(4S)-3-methyl-5,6,7,8-tetrahydro[1,2,4]triazolo[4,3-a]pyrazine | C6 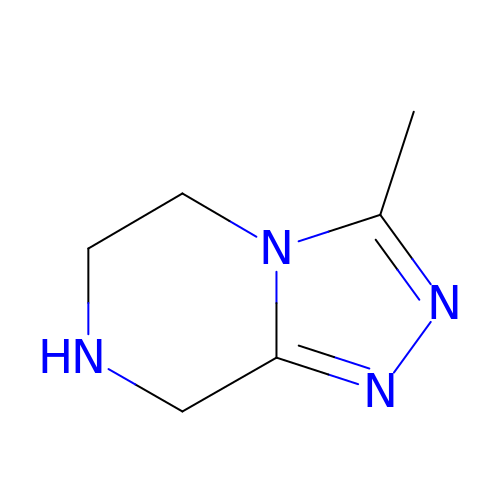H10 N4 | WRGHYZWPWNOJEF-UHFFFAOYSA-N Curli proteins are produced via dedicated and tightly regulated cellular processes, and their fibrils mediate host cell adhesion and invasion, lead to immune system activation, and scaffold bacterial communities known as biofilms. The two key players in curli fibril formation are CsgA and CsgB, the major and minor curli subunits, respectively. CsgA, a 151-residue protein, consists of five imperfect sequence repeats (R1-R5), defined by regularly spaced serine (Ser), glutamine (Gln) and asparagine (Asn) residues. The first and the last repeats (R1 and R5) form amyloid fibrils in isolation and are critical to CsgA seeding and nucleation by CsgB, while the other repeats (R2-R4) contain 'gatekeeper' residues that temper the amyloidogenicity of CsgA.

However, while 45LNIYQY50 (R1), 47IYQYGG52 (R1), and 137VTQVGF142 (R5) formed unbranched and elongated amyloid-like fibrils, the 129TASNSS134 (R4-R5 loop) segment formed scarce and more amorphous structures. The 45LNIYQY50 (R1), 47IYQYGG52 (R1), and 137VTQVGF142 (R5) segments bound the amyloid indicator dye ThT and demonstrated dose-dependent amyloid fibrillation curves with short lag times. 45LNIYQY50 polymerized with the shortest lag time. 45LNIYQY50 and 47IYQYGG52, which are overlapping segments from the R1 repeat, adopted very similar structures. Both segments, as well as 137VTQVGF142 (R5), adopted a classical amyloid steric zipper architecture, with two possible dry interfaces between paired β-sheets. The β-strands were oriented parallel to each other along the β-sheets. These three structures are class 1 steric zippers, as defined by Sawaya and Eisenberg according to the organization of the β-strands and β-sheets. Specifically, the R1 45LNIYQY50 and 47IYQYGG52 segments and the R5 137VTQVGF142 segment formed fibrils that bound the amyloid indicator dye ThT and formed canonical amyloid class 1 steric zippers. These segments contain Gln49 or Gln139 (marked in bold in 45LNIYQY50, 47IYQYGG52, and 137VTQVGF142), which are critical for fibrillation and cannot be mutated to asparagine without interfering with curli assembly. The R1 segment 45LNIYQY50 and the R5 segment 137VTQVGF142 also induced fibrillation of Aβ1–40. In agreement with the hypothesis that the steric zipper segments serve as spines of CsgA fibrils, we found that the D-peptides also inhibited the fibrillation of the R1 45LNIYQY50 and R5 137VTQVGF142 spine segments in a dose-dependent manner.

> LNIYQY3-oxidanylidenepentanoic acid | C5 H8 O3 | 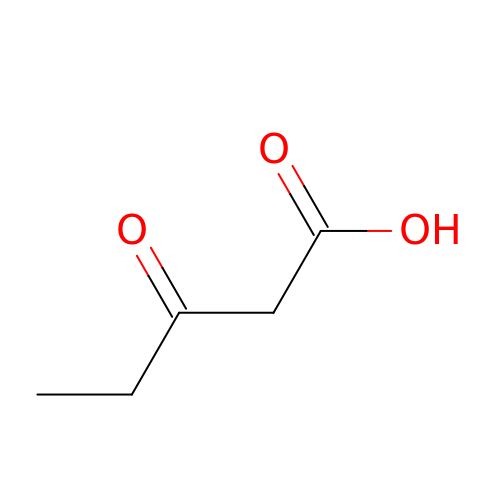FHSUFDYFOHSYHI-UHFFFAOYSA-N> GTGDGSMLSIPPYYRVKNCNLIVDCQYGSTGKGLLAGYLGALEAPQVLCMAPSPNAGHTLVEEDGTARVHKMLPLGITSPSLERIYLGPGSVIDMDRLLEEYLALPRQVELWVHQNAAVVLQEHRDEEAAGGLAPGSTRSGAGSAFIAKIRRRPGTLLFGEAVRDHPLHGVVRVVDTRTAQDMLFRTRSIQAEGCQGYSLSVHHGAYPYCTARDVTTAQLIADCGLPYDVARIARVVGSMRTYPIRVANRPEAGEWSGPCYPDSVECQFADLGLEQEYTTVTKLPRRIFTFSAIQAHEAIAQNGVDEVFLNFAQYPPSLGALEDILDAIEARAEVTYVGFGPKVTDVYHTPTRAELEGLYARYRR

Cyanophage S-2L is known to profoundly alter the biophysical properties of its DNA by replacing all adenines (A) with 2-aminoadenines (Z), which still pair with thymines but with a triple hydrogen bond. It was recently demonstrated that a homologue of adenylosuccinate synthetase (PurZ) and a dATP triphosphohydrolase (DatZ) are two important pieces of the metabolism of 2-aminoadenine, participating in the synthesis of ZTGC-DNA. We now propose a complete 2-aminoadenine metabolic pathway for cyanophage S-2L and related Siphoviridae and Podoviridae phages. The post-infection composition of cellular dNTP pool is heavily altered: dATP is eliminated and replaced by dZTP, which is created in turn from dGTP.

PurZ of cyanophage S-2L and related vibriophage φVC8 from Podoviridae family create the immediate precursor of 2-aminoadenine deoxyribose monophosphate (dZMP), N6-succino-2-amino-2′-deoxyadenylate monophosphate (dSMP), from standard dGMP and free aspartic acid (Asp) using ATP as the energy donor. Here, we determine that S-2L PurZ can use either dATP or ATP as a source of energy, thereby also depleting the pool of nucleotides in dATP. We crystallized S-2L PurZ with two of its substrates, dGMP and dATP, and solved its structure at 1.7 Å resolution. Through crystallographic symmetry, a PurZ dimer can be reconstructed for both S-2L and φVC8. Residues G22, S23, N49, A50, T132, Q190, V241 and the backbone atoms of Y21 form a pocket where the base moiety of dGMP is placed. Y21-S23 are positioned next to the amino group of dGMP in position 2, the hydroxyl group of the conserved S23 being 3.7 Å away from the nitrogen atom. Notably, R146 from the dimer’s other molecule forms an ion pair with the α-phosphate. Like ATP in φVC8 PurZ, the base moiety of dATP is stabilized by stacking interactions with F306 and P336 residues. Oxygen atoms from the side chains of N305, Q308 and the backbone of G335 form hydrogen bonds with adenine’s 6-amino group. The corresponding residues in PurZ extend noticeably further, being 7.9 Å (S-2L R244) and 8.5 Å (φVC8 K267) away from C2′, precluding any possible stabilization of the ribonucleotide.>[4x]SAQSPLLKEQIETIVTGKKATVGVAVWGPDDLEPLLLNPFEKFPMQSVFKLHLAMLVLHQVDQGKLDLNQSVTVNRAAVLQNTWSPMMKDHQGDEFTVAVQQLLQYSVSHSDNVACDLLFELVGGPQALHAYIQSLGVKEAAVVANEAQMHADDQVQYQNWTSMKAAAQV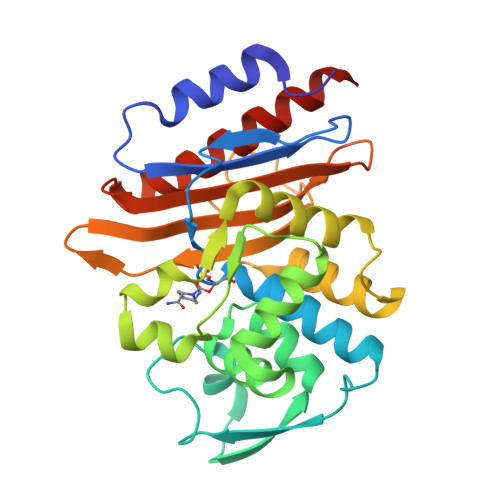LQKFEQKKQLSETSQALLWKWMVETTTGPQRLKGLLPAGTIVAHKTGTSGVRAGKTAATNDAGVIMLPDGRPLLVAVFVKDSAESERTNEAIIAQVAQAAYQFELKKLSAVSPD>[2x]MSLGQLPVVGADGLRPMEQYARPWSGARGTRVAIVVGGLGLSQTGSQKAIRDLPPEVTLGFAASGNSLQRWMQDARREGHEILLQIPLEPFGYPGTNPGPDTLLAGDPAKVNIDRLHRSMAKITNYTGVMNYLGGRFLAEQSALEPVMRDIGKRGLLFLDDGSSAQSLSGGIAKAISAPQGFADVLLDGEVTEASILRKLDD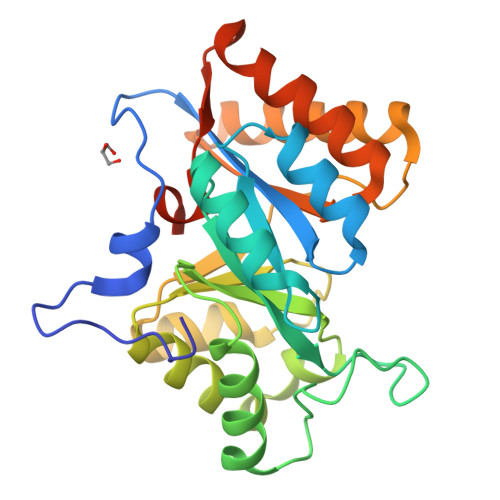LERIARRNGQAIGVASAFDESIAAISKWSREAGGRGIEIVGVSALVSGQAGEGHHHHHH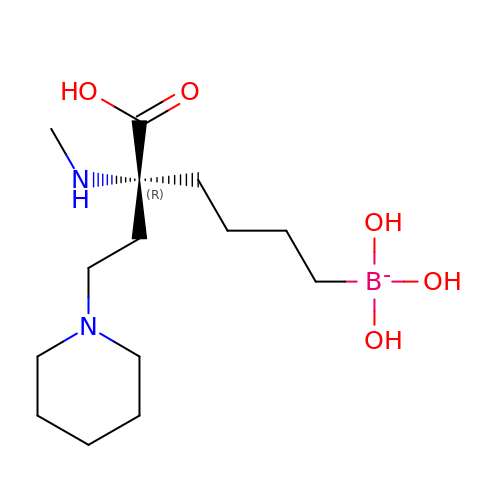[(5R)-5-carboxy-5-(methylamino)-7-(piperidin-1-yl)heptyl](trihydroxy)borate(1-) | C14 H30 B N2 O5 | XUSDRKPOXSYXRQ-CQSZACIVSA-N>GAMASGKVVKFSYMWTINNFSFCREEMGEVIKSSTFSSGANDKLKWCLRVNPKGLDEESKDYLSLYLLLVSCPKSEVRAKFKFSILNAKGEETKAVESQRAYRFVQGKDWGFKKFIRRDFLLDEANGLLPDDKLTLFCEVSVVQD[4x];>[4x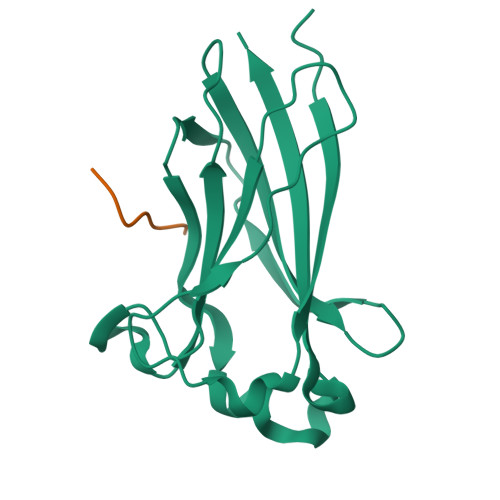]KADTTTPTT RIG-I is an essential innate immune receptor that responds to infection by RNA viruses. The RIG-I signaling cascade is mediated by a series of post-translational modifications, the most important of which is ubiquitination of the RIG-I Caspase Recruitment Domains (CARDs) by E3 ligase Riplet. Riplet is a homodimer composed of an N-terminal RING domain (catalytic domain), CC domain (coiled-coil domain, homodimerization), and C-terminal PrySpry domain (RIG-I recognition domain). Each structure contains two RIG-I molecules, one p3dsRNA24, and one Riplet homodimer, but they differ in the relative positions of two PrySpry domains, which depend on the relative positions of their partner RIG-I molecules.

In the structure composed of the smallest population of particles (6.5%), the second RIG-I is not bound at the opposite terminus at all, but instead binds to a proximal internal duplex site. This results in a head-to-tail arrangement between bound Riplet molecules. Like other internally-bound structures of RIG-I, the CTD is tilted and its conserved diphosphate recognition pocket has melted to accommodate the RNA backbone. This is an interesting result because it suggests that Riplet forms stabilized complexes in cases where two RIG-I molecules are bound on the same RNA, even if there is only one triphosphate end (such as a blunt dsRNA replication intermediate > 20 bp in size). Importantly, we observe that the relative position between the RIG-I molecules is not very important due to flexibility of the Riplet linkers. As the second RIG-I in each structure recognizes different types of RNA sites, the two PrySpry domains bind to RIG-I from different approach angles, revealing variable distances between them, ranging from 58 Å to 101 Å. This finding suggests that the CC domains in these complexes are more dynamic than expected (consistent with our inability to visualize them), enabling the complex to accommodate different spacings between sites of PrySpry domains, and enabling PrySpry domains to approach RIG-I Hel2 from different angles. Despite the different relative orientations of PrySpry in the three structures, the PrySpry domain uses the same interface with RIG-I Hel2 in each case.

>[2x]MTTEQRRSLQAFQDYIRKTLDPTYILSYMAPWFREEEVQYIQAEKNNKGPMEAATLFLKFLLELQEEGWFRGFLDALDHAGYSGLYEAIESWDFKKIEKLEEYRLLLKRLQPEFKTRIIPTDIISDLSECLINQECEEILQICSTKGMMAGAEKLVECLLRSDKENWPKTLKLALEKERNKFSELWIVEKGIKDVETEDLEDKMETSDIQIFYQEDPECQNLSENSCPPSEVSDTNLYSPFKPRNYQLELALPAMKGKNTIICAPTGCGKTFVSLLICEHHLKKFPQGQKGKVVFFANQIPVYEQQKSVFSKYFERHGYRVTGISGATAENVPVEQIVENNDIIILTPQILVNNLKKGTIPSLSIFTLMIFDECHNTSKQHPYNMIMFNYLDQKLGGSSGPLPQVIGLTASVGVGDAKNTDEALDYICKLCASLDASVIATVKHNLEELEQVVYKPQKFFRKVESRISDKFKYIIAQLMRDTESLAKRICKDLENLSQIQNREFGTQKYEQWIVTVQKACMVFQMPDKDEESRICKALFLYTSHLRKYNDALIISEHARMKDALDYLKDFFSNVRAAGFDEIEQDLTQRFEEKLQELESVSRDPSNENPKLEDLCFILQEEYHLNPETITILFVKTRALVDALKNWIEGNPKLSFLKPGILTGRGKTNQNTGMTLPAQKCILDAFKASGDHNILIATSVADEGIDIAQCNLVILYEYVGNVIKMIQTRGRGRARGSKCFLLTSNAGVIEKEQINMYKEKMMNDSILRLQTWDEAVFREKILHIQTHEKFIRDSQEKPKPVPDKENKKLLCRKCKALACYTADVRVIEECHYTVLGDAFKECFVSRPHPKPKQFSSFEKRAKIFCARQNCSHDWGIHVKYKTFEIPVIKIESFVVEDIATGVQTLYSKWKDFHFEKIPFDPAEMSK;>MAGLGLGSAVPVWLAEDDLGCIICQGLLDWPATLPCGHSFCRHCLEALWGARDARRWACPTCRQGAAQQPHLRKNTLLQDLADKYRRAAREIQAGSDPAHCPCPGSSSLSSAAARPRRRPELQRVAVEKSITEVAQELTELVEHLVDIVRSLQNQRPLSESGPDNELSILGKAFSSGVDLSMASPKLVTSDTAAGKIRDILHDLEEIQEKLQESVTWKEAPEAQMQGELLEAPSSSSCPLPDQSHPALRRASRFAQWAIHPTFNLKSLSCSLEVSKDSRTVTVSHRPQPYRWSCERFSTSQVLCSQALSSGKHYWEVDTRNCSHWAVGVASWEMSRDQVLGRTMDSCCVEWKGTSQLSAWHMVKETVLGSDRPGVVGIWLNLEEGKLAFYSVDNQEKLLYECTISASSPLYPAFWLYGLHPGNYLIIKQVKV[2x]1-[1-[2,5-dimethoxy-4-[(1~{S})-1-oxidanylethyl]phenyl]indolizin-3-yl]ethanone 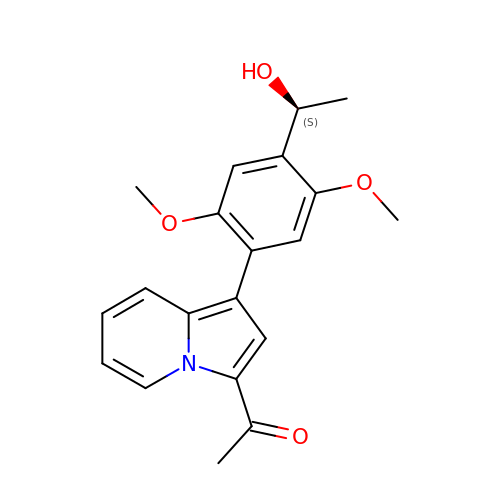| C20 H21 N O4 | HZDNKVMOCMTBLZ-LBPRGKRZSA-N>MTATSDKVLKIQLRSASATVPTKGSATAAGYDIYASQDITIPAMGQGMVSTDISFTVPVGTYGRIAPRSGLAVKNGIQTGAGVVDRDYTGEVKVVLFNHSQRDFAIKKGDRVAQLILEKIVDDAQ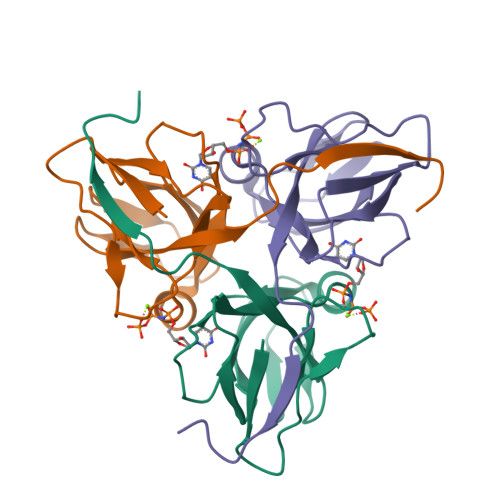IVVVDSLEESARGAGGFGSTGN[3x]> MGNLYSSLPLTKREEVEKLLNGDTWRHLAGELGYQPEHIDSFTHEACPVRALLASWGAQDSA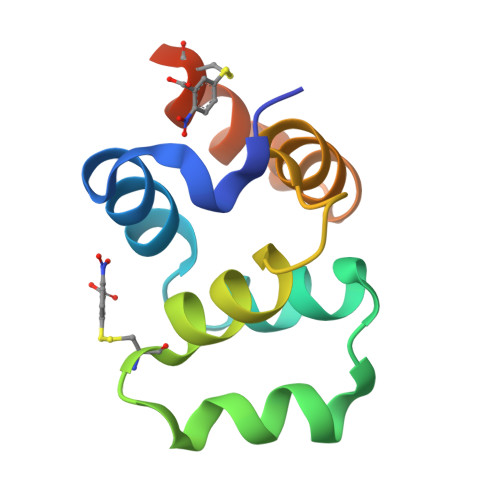TLDALLAALRRIQRADIVESLCSELEHHHHHH>MAISKRHIGPYIIRETLGEGSFGKVKLATHYKTQQKVALKFISRQLLKKSDMHMRVEREISYLKLLRHPHIIKLYDVITTPTDIVMVIEYAGGELFDYIVEKKRMTEDEGRRFFQQIICAIEYCHRHKIVHRDLKPENLLLDDNLNVKIADFGLSNIMTDGNFLKTSCGSPNYAAPEVINGKLYAGPEVDVWSCGIVLYVMLVGRLPFDDEFIPNLFKKVNSCVYVMPDFLSPGAQSLIRRMIVADPMQRITIQEIRRDPWFNVNLPDYLRPMEEVQGSYADSRIVSKLGEAMGFSEDY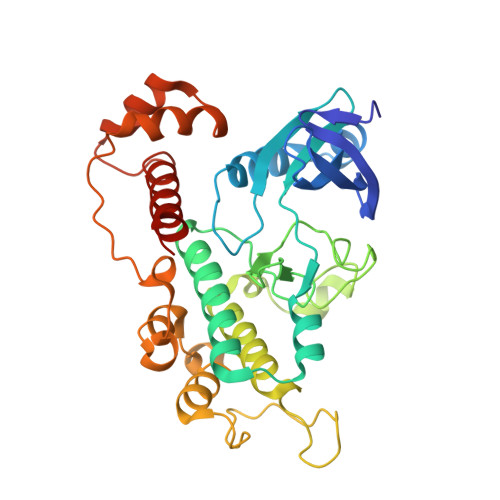IVEALRSDENNEVKEAYNLLHENQVIQEKLEHHHHHH[2x]>[60x]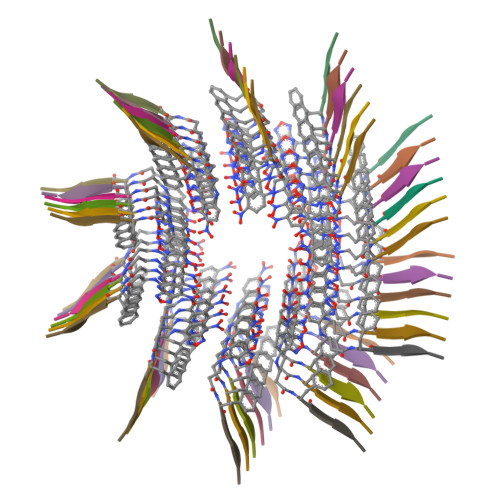XFFSY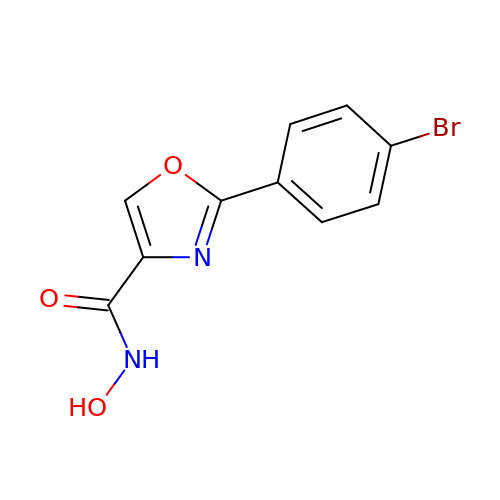2-(4-bromophenyl)-N-hydroxy-1,3-oxazole-4-carboxamide | C10 H7 Br N2 O3 | KHPRTOQUGAUDCM-UHFFFAOYSA-N> GPESAPRIMRLVAECSRSGARAGELRLPHGTVATPVFMPVGTQATMKGITTEQLDSLGCRICLGNTYHLGLRPGPELIRKAQGLHGFMNWPHNLLTDSGGFQMVSLFSLSEVTEEGVHFRSPYDGEETLLSPERSVEIQNALGSDIIMQLDHVVSSTVTGPLVEEAMHRSVRWLDRCIAAHKHPDKQNLFAIIQGGLNADLRTTCLKEMTKRDVPGFAIGGLSGGESKAQFWKMVALSTSMLPKDKPRYLMGVGYATDLVVCVALGCDMFDCVYPTRTARFGSALVPTGNLQLKKKQYAKDFSPINPECPCPTCQTHSRAFLHALLHSDNTTALHHLTVHNIAYQLQLLSAVRSSILEQRFPDFVRNFMRTMYGDHSLCPAWAVEALASVGIMLT;> GPKLSLIKVVNGCRLGKIQNLGKAGDCTVDIPGCLLYTRTGSAPHLTHQTLRNIHGVPGIAQLTLSSLAEHHEVLAEYKKGVGSFIGMPESLFYCSLHDPVTPGPAGYVTSKSVSVWGFGGRVEMTVSKFMAIQEALQPDWFQCLSDGEASCAETTSIKRARKSVDRSLLFLDSCLRLQEESEVLQKSVIIGVIEGGDVMEERLRSARETAKRPVGGFLLDGFQGDPAVTETRLHLLSSVTAELPEDKPRLICGVSRPDEVLECIERGVDLFESFFPYQVTERGCALTFTFDCQLNPEETLLQQNGIQEKIKGLDQAKKIEATGCNQEMTSFEINLKEKKYQEDFDPLVRGCSCYCCKNHTRAYIHHLLMTNELLAGVLLMMHNFEHYFGFFCSIREALKNDTLAQLKE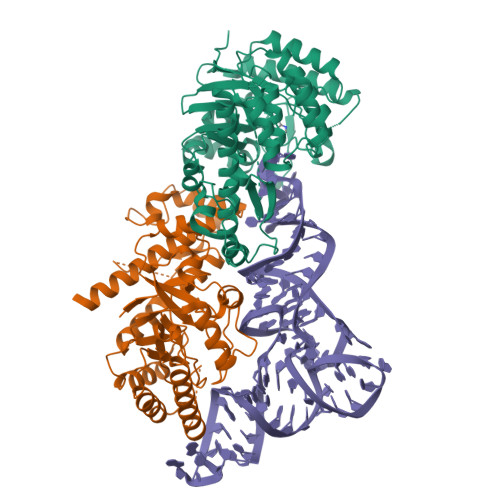LICRQMF>[2x]MMEQVCDVFDIYAICACCKVESKNEGKKNEVFNNYTFRGLGNKGVLPWKCNSLDMKYFRAVTTYVNESKYEKLKYKRCKYLNKETVDNVNDMPNSKKLQNVVVMGRTNWESIPKKFKPLSNRINVILSRTLKKEDFD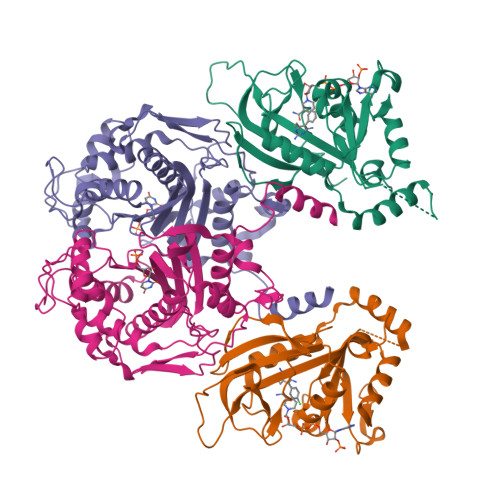EDVYIINKVEDLIVLLGKLNYYKCFIIGGSVVYQEFLEKKLIKKIYFTRINSTYECDVFFPEINENEYQIISVSDVYTSNNTTLDFIIYKKTNNKMLNEQNCIKGEEKNNDMPLKNDDKDTCHMKKLTEFYKNVDKYKINYEN;>[2x]DDDDEEEDDFVYFNFNKEKEEKNKNSIHPNDFQIYNSLKYKYHPEYQYLNIIYDIMMNGNKQSDRTGVGVLSKFGYIMKFDLSQYFPLLTTKKLFLRGIIEELLWFIRGETNGNTLLNKNVRIWEANGTREFLDNRKLFHREVNDLGPIYGFQWRHFGAEYTNMYDNYENKGVDQLKNIINLIKNDPTSRRILLCAWNVKDLDQMALPPCHILCQFYVFDGKLSCIMYQRSCDLGLGVPFNIASYSIFTHMIAQVCNLQPAQFIHVLGNAHVYNNHIDSLKIQLNRIPYPFPTLKLNPDIKNIEDFTISDFTIQNYVHHEKISMDMAA N-carbamoyl-L-methionine | C6 H12 N2 O3 S | 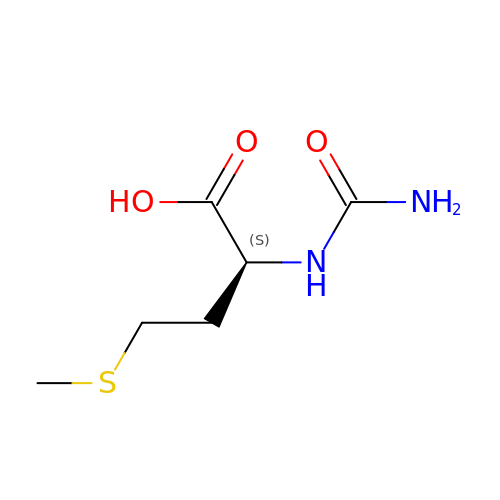DEWDMTSMCKXBNP-BYPYZUCNSA-N>[2x]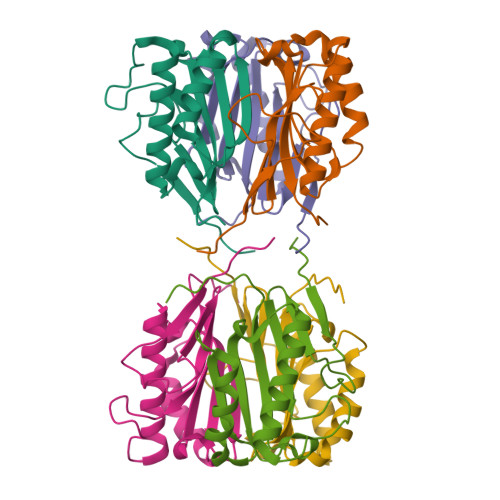GSHMSSLVRRIISTAKAPAAIGPYSQAVLVDRTIYISGQLGMDPASGQLVPGGVVEEAKQALTNIGEILKAAGCDFTNVVKATVLLADINDFSAVNDVYKQYFQSSFPARAAYQVAALPKGGRVEIAAIAVQGPLTTASL>XGPPGPPGPPGXPGPPGPPGPPX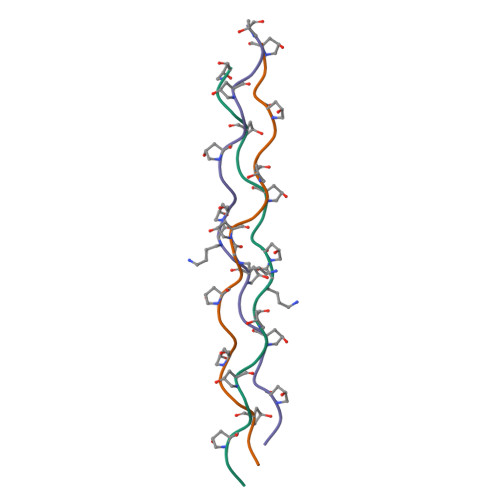[3x]>MGDSEVDKAVSLVEELAQKSGSENAREAAKEIRKRGDSEVALAVALVLSLANKSGSRNAIEAAAEIAKRGDSEVALAVALVLSLANKSGSRNAIEAAAEIAKRGDSEVALAVALVLSLANKSGSRNAIEAAAEIAKRGDSEVALAVALVLSLANKSGSRNAIEAAAEIAKRGDSEVALAVALVLSLANKSGSRNAIEAAAEIA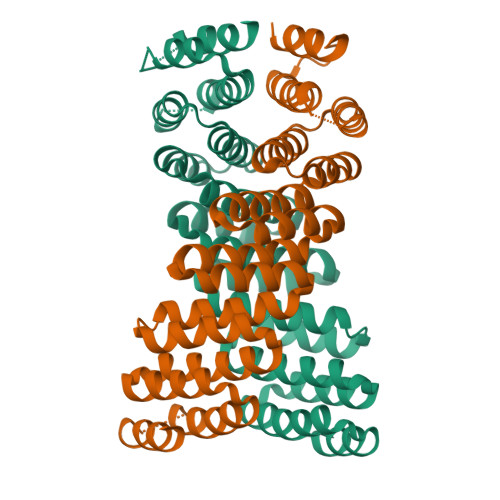KRGDSEVALAVALVLSLANKSGSRNAIEAAAEIAKRGDSEVALKVALELSQANKNGSRDEIEKAAENAKRGDGWLEHHHHHH[2x]>[2x]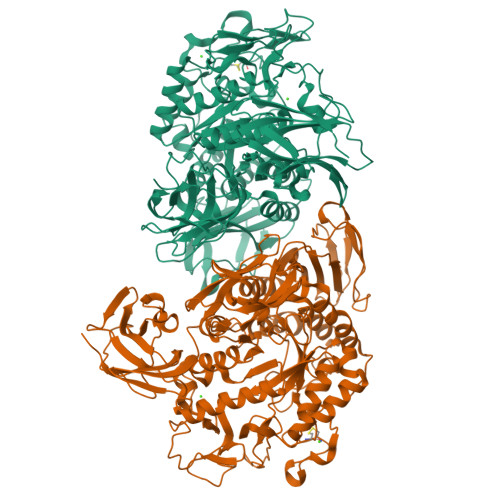APDTSVSNKQNFSTDVIYQIFTDRFSDGNPANNPTGAAFDGSCTNLRLYCGGDWQGIINKINDGYLTGMGITAIWISQPVENIYSVINYSGVNNTAYHGYWARDFKKTNPAYGTMQDFKNLIDTAHAHNIKVIIDFAPNHTSPASSDDPSFAENGRLYDNGNLLGGYTNDTQNLFHHYGGTDFSTIENGIYKNLYDLADLNHNNSSVDVYLKDAIKMWLDLGVDGIRVDAVKNMPFGWQKSFMATINNYKPVFTFGEWFLGVNEISPEYHQFANESGMSLLDFRFAQKARQVFRDNTDNMYGLKAMLEGSEVDYAQVNDQVTFIDNHDMERFHTSNGDRRKLEQALAFTLTSRGVPAIYYGSEQYMSGGNDPDNRARLPSFSTTTTAYQVIQKLAPLRKSNPAIAYGSTHERWINNDVIIYERKFGNNVAVVAINRNMNTPASITGLVTSLPRGSYNDVLGGILNGNTLTVGAGGAASNFTLAPGGTAVWQYTTDATTPIIGNVGPMMAKPGVTITIDGRGFGSGKGTVYFGTTAVTGADIVAWEDTQIQVKIPAVPGGIYDIRVANAAGAASNIYDNFEVLTGDQVTVRFVINNATTALGQNVFLTGNVSELGNWDPNNAIGPMYNQVVYQYPTWYYDVSVPAGQTIEFKFLKKQGSTVTWEGGANRTFTTPTSGTATVNVNWQP> GIDPFTAKRTHRVINHPYYFPFNGRQAEDYLRSKERGEFVIRQ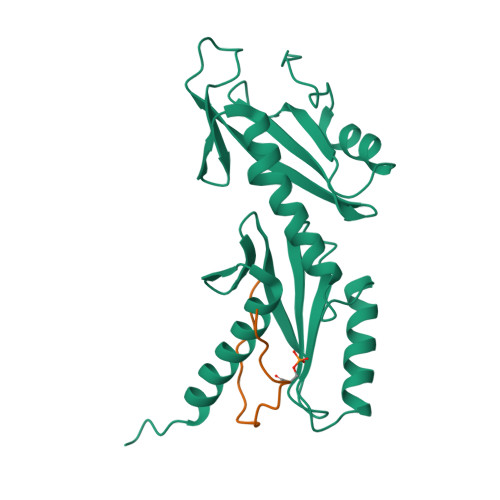SSRGDDHLVITWKLDKDLFQHIDIQELEKENPLALGKVLIVDNQKYNDLDQIIVEYLQNKVRLLNEMTSSEKFKSGTKKDVVKFIEDYSRVNPNKSVYYFSLNHDNPGWFYLMFKINANSKLYTWNVKLTNTGYFLVNYNYPSVIQLCNGFKTLLKSNSSKNRMNNYR;> ESGLVNADLDVKDELMFSPLVDS> GIPMAVTITLKTLQQQTFKIRMEPDETVKVLKEKIEAEKGRDAFPVAGQKLIYAGKI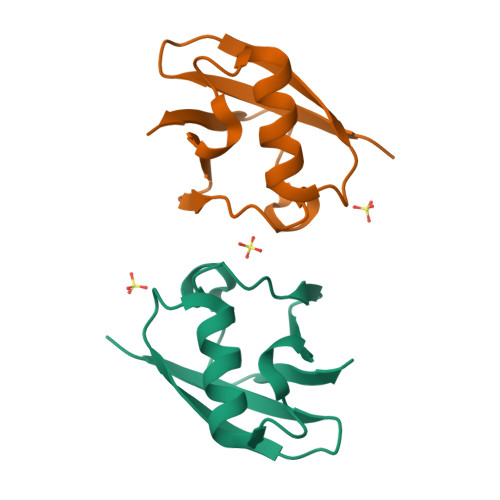LSDDVPIRDYRIDEKNFVVVMVTKTKAG>MGSSHHHHHHHHHHSSGLVPRGSHMTGHSNGQDLVMKANEKYLVKNAQQPERGKIYDRNGKVLAEDVERYKLVAVIDKKASANSKKPRHVVDKKETAKKLSTVIDMKPEEIEKRLSQKKAFQIEFGRKGTNLTYQDKLKIEKMNLPGISLLPETERFYPNGNFASHLIGRAQKNPDTGELKGALGVEKIFDSYLSGSKGSLRYIHDIWGYIAPNTKKEKQPKRGDDVHLTIDSNIQVFVEEALDGMVERYQPKDLFAVVMDAKTGEILAYSQRPTFNPETGKDFGKKWANDLYQNTYEPGSTFKSYGLAAAIQEGAFDPDKKYKS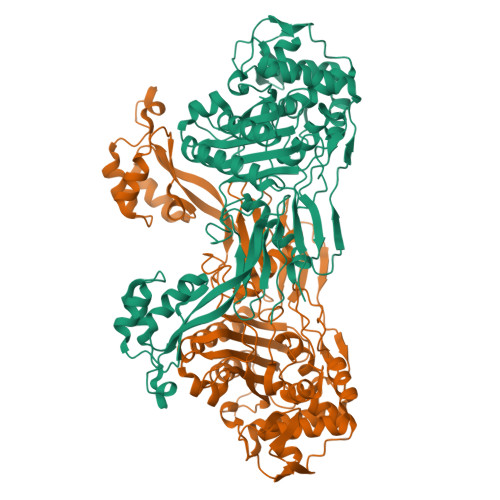GHRDIMGSRISDWNRVGWGEIPMSLGFTYSSNTLMMHLQDLVGADKMKSWYERFGFGKSTKGMFDGEAPGQIGWSNELQQKTSSFGQSTTVTPVQMLQAQSAFFNDGNMLKPWFVNSVENPVSKRQFYKGQKQIAGKPITKDTAEKVEKQLDLVVNSKKSHAANYRIDGYEVEGKTGTAQVAAPNGGGYVKGPNPYFVSFMGDAPKKNPKVIVYAGMSLAQKNDQEAYELGVSKAFKPIMENTLKYLNVGKSKDDTSNAEYSKVPDVEGQ[2x]N-hydroxy-7-sulfanylheptanamide | C7 H15 N O2 S | 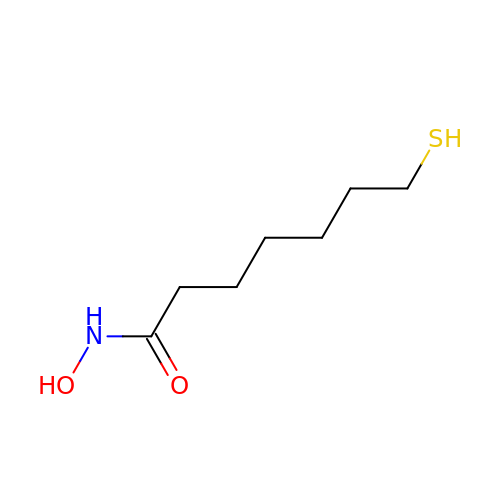XKCHGAJRKPXTNT-UHFFFAOYSA-N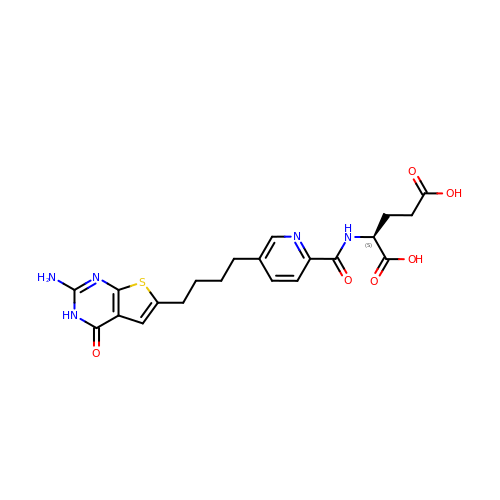N-{5-[4-(2-amino-4-oxo-3,4-dihydrothieno[2,3-d]pyrimidin-6-yl)butyl]pyridine-2-carbonyl}-L-glutamic acid | C21 H23 N5 O6 S | BKEFFQOOMQZMDH-HNNXBMFYSA-N>[2x]MATATEQWVLVEMVQALYEAPAYHLILEGILILWIIRLLFSKTYKLQERSDLTVKEKEELIEEWQPEPLVPPVPKDHPA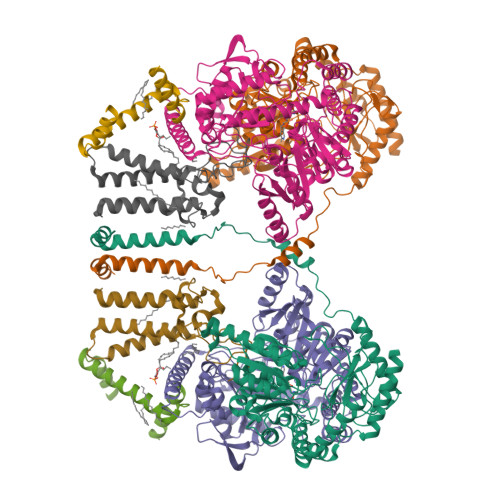LNYNIVSGPPSHKTVVNGKECINFASFNFLGLLDNPRVKAAALASLKKYGVGTCGPRGFYGTFDVHLDLEDRLAKFMKTEEAIIYSYGFATIASAIPAYSKRGDIVFVDRAACFAIQKGLQASRSDIKLFKHNDMADLERLLKEQEIEDQKNPRKARVTRRFIVVEGLYMNTGTICPLPELVKLKYKYKARIFLEESLSFGVLGEHGRGVTEHYGINIDDIDLISANMENALASIGGFCCGRSFVIDHQRLSGQGYCFSASLPPLLAAAAIEALNIMEENPGIFAVLKEKCGQIHKALQGISGLKVVGESLSPAFHLQLEESTGSREQDVRLLQEIVDQCMNRSIALTQARYLEKEEKCLPPPSIRVVVTVEQTEEELERAASTIKEVAQAVLL;>MRPEPGGCCCRRTVRANGCVANGEVRNGYVRSSAAAAAAAAAGQIHHVTQNGGLYKRPFNEAFEETPMLVAVLTYVGYGVLTLFGYLRDFLRYWRIEKCHHATEREEQKDFVSLYQDFENFYTRNLYMRIRDNWNRPICSVPGARVDIMERQSHDYNWSFKYTGNIIKGVINMGSYNYLGFARNTGSCQEAAAKVLEEYGAGVCSTRQEIGNLDKHEELEELVARFLGVEAAMAYGMGFATNSMNIPALVGKGCLILSDELNHASLVLGARLSGATIRIFKHNNMQSLEKLLKDAIVYGQPRTRRPWKKILILVEGIYSMEGSIVRLPEVIALKKKYKAYLYLDEAHSIGALGPTGRGVVEYFGLDPEDVDVMMGTFTKSFGASGGYIGGKKELIDYLRTHSHSAVYATSLSPPVVEQIITSMKCIMGQDGTSLGKECVQQLAENTRYFRRRLKEMGFIIYGNEDSPVVPLMLYMPAKIGAFGREMLKRNIGVVVVGFPATPIIESRARFCLSAAHTKEILDTALKEIDEVGDLLQLKYSRHRLVPLLDRPFDETTYEETED[2x];>[2x]MAGMALARAWKQMSWFYYQYLLVTALYMLEPWERTVFNSMLVSIVGMALYTGYVFMPQHIMAILHYFEIVQ;>MNVGTAHSEVNPNTRVMNSRGIWLSYVLAIGLLHIVLLSIPFVSVPVVWTLTNLIHNMGMYIFLHTVKGTPFETPDQGKARLLTHWEQMDYGVQFTASRKFLTITPIVLYFLTSFYTKYDQIHFVLNTVSLMSVLIPKLPQLHGVRIFGINKY[2x]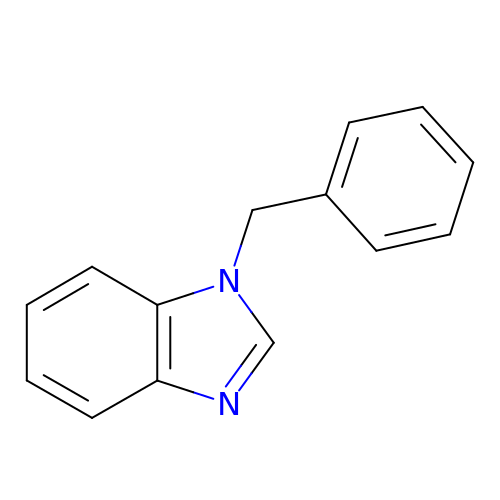1-benzyl-1H-benzimidazole | C14 H12 N2 | MNEIJGDSFRHGMS-UHFFFAOYSA-N>AAAKPATTEGEFPETREKMSGIRRAIAKAMVHSKHTAPHVTLMDEADVTKLVAHRKKFKAIAAEKGIKLTFLPYVVKALVSALREYPVLNTSIDDETEEIIQKHYYNIGIAADTDRGLLVPVIKHADRKPIFALAQEINELAEKARDGKLTPGEMKGASCTITNIGSAGGQWFTPVINHPEVAILGIGRIAEKPIVRDGEIVAAPMLALSLSFDHRMIDG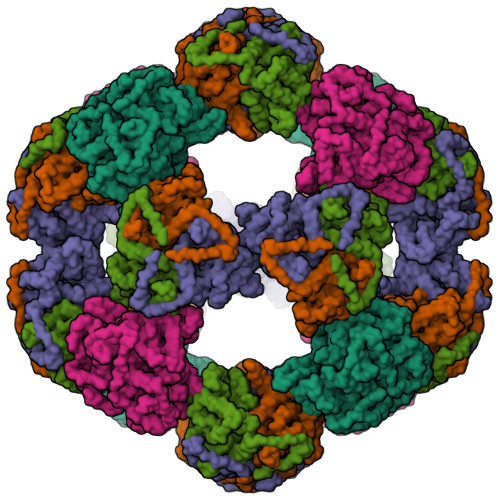ATAQKALNHIKRLLSDPELLLM[5x]[1,1,1-tris(fluoranyl)-2-methyl-propan-2-yl] ~{N}-[(1~{S},4~{R},6~{S},7~{Z},11~{R},13~{R},14~{S},18~{R})-13-ethyl-18-(7-fluoranyl-6-methoxy-isoquinolin-1-yl)oxy-11-methyl-4-[(1-methylcyclopropyl)sulfonylcarbamoyl]-2,15-bis(oxidanylidene)-3,16-diazatricyclo[14.3.0.0^{4,6}]nonadec-7-en-14-yl]carbamate 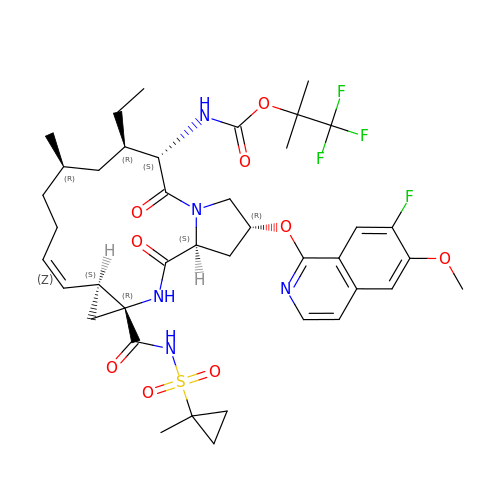| C40 H51 F4 N5 O9 S | IJNUZTYJYYUXSD-SMNGPBTOSA-N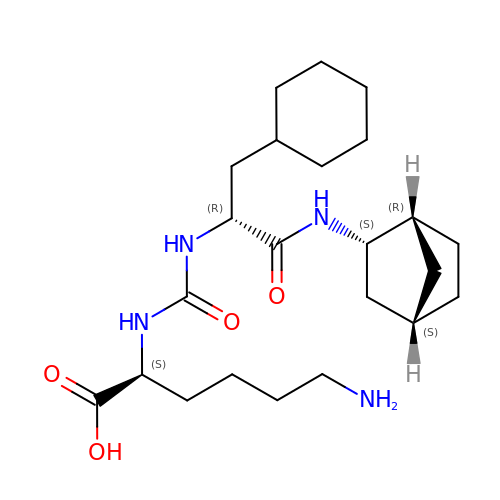(2~{S})-6-azanyl-2-[[(2~{R})-1-[[(1~{R},2~{S},4~{S})-2-bicyclo[2.2.1]heptanyl]amino]-3-cyclohexyl-1-oxidanylidene-propan-2-yl]carbamoylamino]hexanoic acid | C23 H40 N4 O4 | HKPGTWCJLYFZSN-LJDSDSDDSA-N>[2x]SGGYAVDYSEPIIIKEKGEIKVVKIGELIDEIIKNSKNVRKDGILEIARCKDVEVIAFDSNYKFKFMPVSEVSRHPVSEMFEIVVEGNKKVRVTGSHSVFTVKDNEVV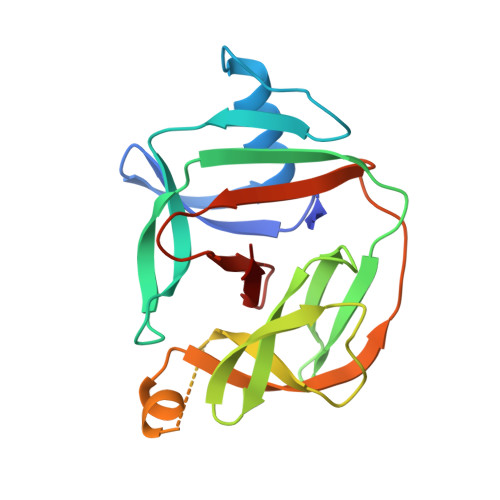PIRVDDLRVGDILVLAKELPNIEENRKLEPNIEENRKLEKLINSDFIFLKIKKINKVEPTNGYAYDLTVPNAENFIAGFGGFVLHNA>AATDALTGVANRRMLDQSLRHEWFRAQRSGKPLSLLMIDADHFKAFNDRHGHQAGDQALRELARVITTNVRRPADLVARYGGEEFSVILAETDSVGAQQIAEHIRAAVEQLSSVNEDQSPMTVSIGISTWTATSEISLEQLLFAADKALYQAKEGGRNRVVVAALEHHHHHH[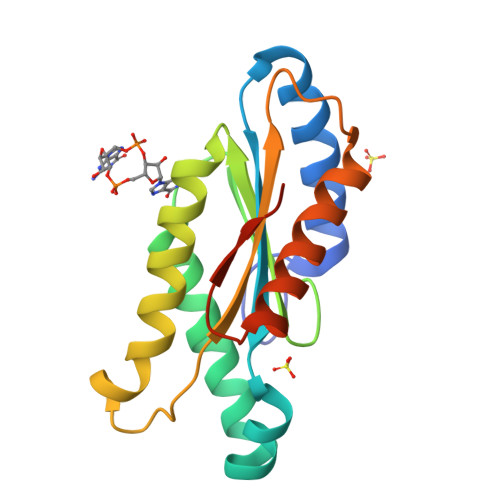4x]>[2x]MASQPNSSAKKKEEKGKN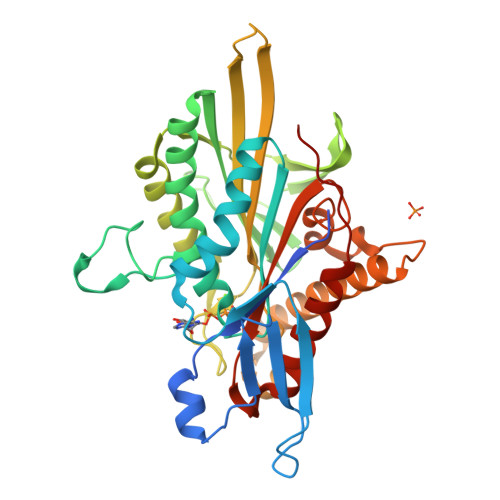IQVVVRCRPFNLAERKASAHSIVECDPVRKEVSVRTGGLADKSSRKTYTFDMVFGASTKQIDVYRSVVCPILDEVIMGYNCTIFAYGQTGTGKTFTMEGERSPNEEYTWEEDPLAGIIPRTLHQIFEKLTDNGTEFSVKVSLLEIYNEELFDLLNPSSDVSERLQMFDDPRNKRGVIIKGLEEITVHNKDEVYQILEKGAAKRTTAATLMNAYSSRSHSVFSVTIHMKETTIDGEELVKIGKLNLVDLAGSENIGRSGAVDKRAREAGNINQSLLTLGRVITALVERTPHVPYRESKLTRILQDSLGGRTRTSIIATISPASLNLEETLSTLEYAHRAKNILNKPEVNQKL>FACKTANGTAIPIGGGSANVYVNLAPAVNVGQNLVVDLSTQIFCHNDYPETITDYVTLQRGSAYG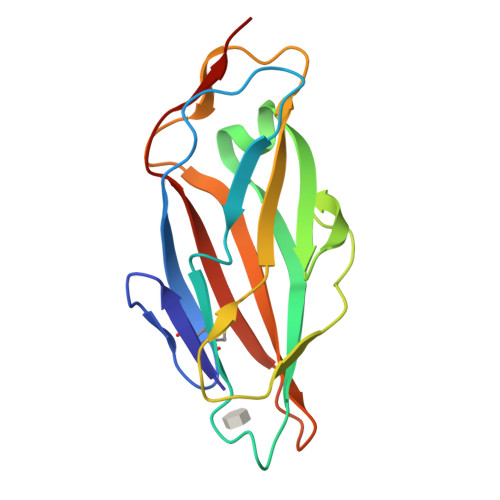GVLSSFSGTVKYNGSSYPFPTTSETPRVVYNSRTDKPWPVALYLTPVSSAGGVAIKAGSLIAVLILRQTNNYNSDDFQFVWNIYANNDVVVPTG[2x]~{N}-[(2~{R},3~{R},4~{S},5~{S},6~{R})-6-(hydroxymethyl)-3,4,5-tris(oxidanyl)oxan-2-yl]-4-phenyl-benzamide | C19 H21 N O6 | 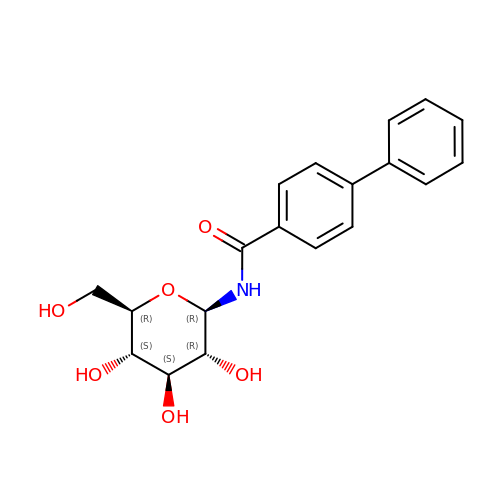FEGAJDJNSVSMNR-OGJJZOIMSA-N>SNAGNSTTSDKGTEEATTSAFDVMSQFNEIGVSYPLTVTDQAGRTVTFEKAPEKIASSYYISTSLLLALGLQDKLVGIEAKANTRNIYKLAAPAIVSLPNMGTAKEFNTEACVAATPDVVFLPMKLKKTADTLESLGIKAVVVNPEDQSLLEECITLVGKITNNAGRAEALNNSIKTFLADNKTNVSGGNTPSVYLAGNSSVLSTAGSKMYQNTLLTNAGGKNVASELTDTYWANVSYEQILAWNPDYIVIAADATYTVDDILNDANLAGCNAVKNKNVVKLPNNIEAWDS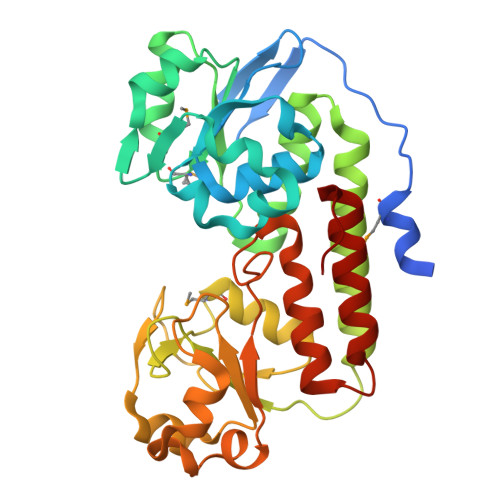PVPGSFLGSIYIASVLHPEKVTKDFYETCVTKFYESFYGFTPAK[2x]> AHNNENVSGISAYLLGLIIGDGGLYKLKYKGNRSEY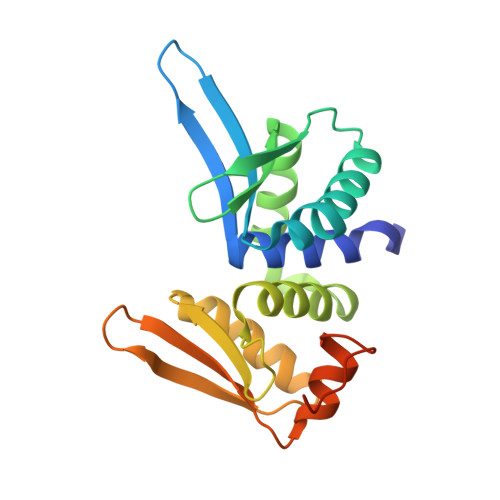RVVITQKSENLIKQHIAPLMQFLIDELNVKSKIQIVKGDTRYELRVSSKKLYYYFANMLERIRLFNMREQIAFIKGLYVAEGDKTLKRLRIWNKNKALLEIVSRWLNNLGVRNTIHLDDHRHGVYVLNISLRDRIKFVHTILSSHLNPLPPEAAALEHHHHHH>[4x]SYTLPSLPYAYDALEPHFDKQTMEIHHTKHHQTYVNNANAALESLPEFANLPVEELITKLDQLPADKKTVLRNNAGGHANHSLFWKGLKKGTTLQGDLKAAIERDF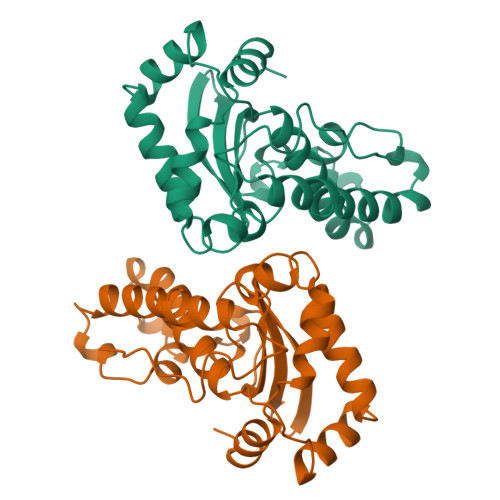GSVDNFKAEFEKAAASRFGSGWAWLVLKGDKLAVVSTANQDSPLMGEAISGASGFPIMGLDVWEHAYYLKFQNRRPDYIKEFWNVVNWDEAAARFAAKK> GSHMASMTGGQQMGRGSMLPRLICINDYEQHAKSVLPKSIYDYYRSGANDEETLADNIAAFSRWKLYPRMLRNVAETDLSTSVLGQRVSMPICVGATAMQRMAHVDGELATVRACQSLGTGMMLSSWATSSIEEVAEAGPEALRWLQLYIYKDREVTKKLVRQ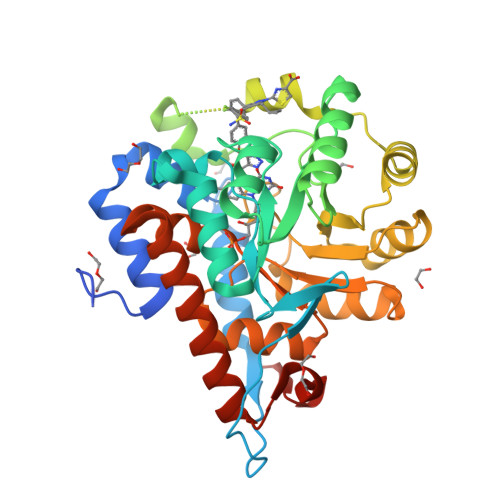AEKMGYKAIFVTVDTPYLGNRLDDVRNRFKLPPQLRMKNFETSTLSFSPEENFGDDSGLAAYVAKAIDPSISWEDIKWLRRLTSLPIVAKGILRGDDAREAVKHGLNGILVSNHGARQLDGVPATIDVLPEIVEAVEGKVEVFLDGGVRKGTDVLKALALGAKAVFVGRPIVWGLAFQGEKGVQDVLEILKEEFRLAMALSGCQNVKVIDKTLVRKNPLAVSKI> MKFSNITIKNFRNFEKVNINLDNKNVIFGMNDIGKTNFLYALRFLLDKEIRKFGFNKSDYHKHDTSKKIEIILTLDLSNYEKDEDTKKLISVVKGARTSANADVFYIALESKYDDKELYGNIILKWGSELDNLIDIPGRGNINALDNVFKVIYINPLVDLDKLFAQNKKYIFEESQG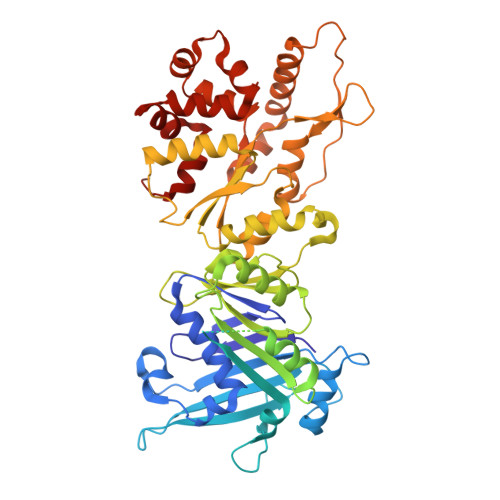NESDEGILNNIKSLTDQVNQQIGEMTIIKGFQQEITSEYRSLKKEEVSIELKSEMAIKGFFSDIIPYIKKDGDSNYYPTSGDGRRKMLSYSIYNYLAKKKYEDKIVIYLIEEPEISLHRSMQIALSKQLFEQSTYKYFFLSTHSPELLYEMDNTRLIRVHSTEKVVCSSHMYNVEEAYGSVKKKLNKALSSALFAERVLLIEGPSEKILFEKVLDEVEPEYELNGGFLLEVGGTYFNHYVCTLNDLGITHIIKTDNDLKSKKGKKGVYELLGLNRCLNLLGRENLDEITIDIPEDIKGKKKKERLNERKKEIFKQYKNEVGEFLGERIYLSEIDLENDLYSAIGESMKRIFENEDPVHYLQKSKLFNMVELVNNLSTKDCFDVFEHEKFACLKELVGSDRG TodS/TodT, a two-component signal transduction system, is responsible for regulation of tod operon expression in P. putida strains. TodS lacks a transmembrane region, and its N-terminal PAS domain (PAS1) binds a wide range of effectors, including toluene, to trigger increased basal autophosphorylation of TodS, leading to a phospho-signal relay to TodT and ultimately transcriptional stimulation of the tod operon genes by interacting with phosphorylated TodT in the PtodX promoter region (11–14). In the present study, we determined the crystal structures of the TodS PAS1 domain in complex with either toluene (an agonist) or 1,2,4-trimethylbenzene (1,2,4-TMB; an antagonist), as well that of apo-PAS1. The structure of each PAS1 domain is very similar to those described for other PAS domain structures, which consist of a five-stranded antiparallel β-sheet and three α-helices spanning residues 45–149.

There are two PAS1 molecules in each asymmetric unit, resulting in an antiparallel dimer structure. An additional α-helix (α4, residues 150–163) is located immediately outside the canonical PAS fold in molecule A. Remarkably, the corresponding region of α4 is completely disordered in molecule B. The TodS PAS1 domain constructed in this study did not include the corresponding helix region; thus, the antiparallel face-to-face dimerization observed in the TodS PAS1 structure may be an artificial consequence of the symmetry of crystal packing. During refinement of the apo-PAS1 structure, we noted a region of weak electron density in the hydrophobic ligand-binding pocket. The shape of the region is somewhat similar to those of benzene-derived compounds, including toluene and 1,2,4-TMB. Thus, we thought that the region of weak electron density observed in the apo-PAS1 structure may have originated from contaminants in the incubator (or the laboratory environment). It may also be possible that a cellular ligand, such as an aromatic compound, was co-purified with PAS1 protein. In the absence of a signal effector, the PAS1 sensor domain cannot provide a signal to HK1 via the flexible nature of the STR. This conformation cannot induce the functional dimeric conformation of HK1 to enable autophosphorylation.

>[2x]GAMALYEFVGLLDAHGNVLEVNQVALEGGGITLEEIRGKPFWKARWWQISKKTEATQKRLVETASSGEFVRCDVEILGKSGGREVIAVDFSLLPICNEEGSIVYLLAEGRNITDKKKAEAMLALKNQELE> GPHMIHSSVKRWGNSPAVRIPATLMQALNLNIDDEVKIDLVDGKLIIEPVRKEPVFTLAELVNDITPE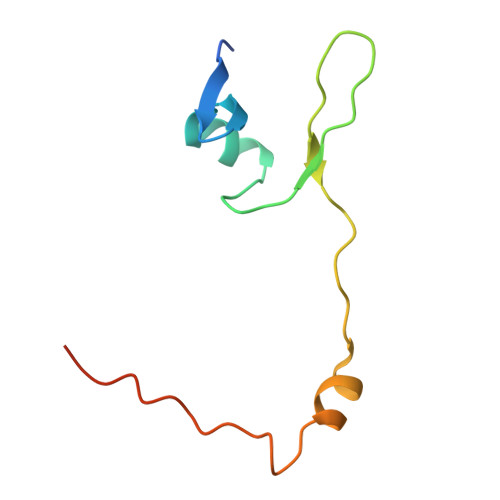NLHENIDWGEPKDKEVW>MRYGHFDDEAREYVITTPHTPYPWINYLGSEQFFSLLSHQAGGYSFYRDAKMRRLTRYRYNNIPADAGGRYLYVNDGGDVWTPSWLPVKADLDHFEARHGLGYSTITGERNGVRVETLFFVPVGENAEVQKVTVTNTSDSYKSLTLFSFVEFCLWNAQDDQTNYQRNLSIGEVEVEQESPHGSAIYHRTEYRERRDHYAVFAVNTQAEGFDTDRDTFVGAYNSLGEAAVPLKGESANSVASGWYPIGSHSVAVSLAPGESRELVYVLGYVENPDEEKWADDAKQVVNKERAHALLSRFATSEQTDAAFAALKDYWTDLLSTYSVSSNDEKLDRMVNIWNQYQCMVTFNMSRSASFFETGIGRGMGFRDSNQDLLGFVHLIPERARERIIDIASTQFADGSAYHQYQPLTKRGNNDIGSGFNDDPLWLIAGTAAYIKETGDFSILDEPVPFDNEPGSEVPLFEHLTRSFEFTVTHRGPHGLPLIGRADWNDCLNLNCFSTTPGESFQTTENQAGGVAESTFIAAQFVLYGEQYAELAARRGLADVADRARGHVAEMRDALLTDGWDGSWFLRAYDYYGNPIGTDAHDEGKIWIEPQGFAVMAGVGVGEGPQDTDAPAIKALDSVNEMLATDHGMVLQYPAYTTYQVHMGEVSTYPPGYKENGGIFCHNNPWVIIAETVVGRGGRAFDYYKR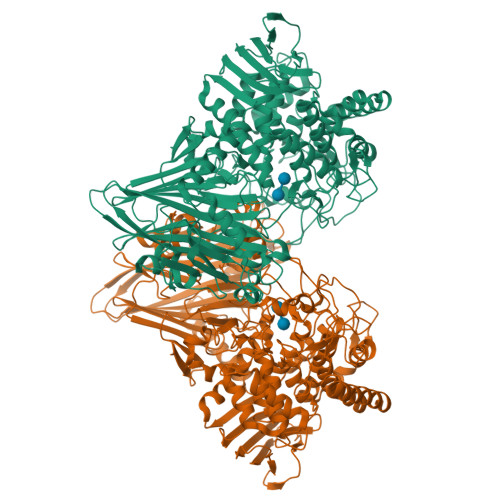ITPAYREDISDVHRLEPYVYAQMIAGKEAVRHGEAKNSWLTGTAAWNFVTVSQYLLGVRPEYDGLVVDPQIGPDVPSFTVTRVARGATYEITVTNSGTDGSRGRLVVDGTPVEGNLVPYAPAGSTVRVDVTL[2x]> MVKETHRFETFTEEPIRLIGEEGEWLGDFPLDLEGEKLRRLYRDMLAARMLDERYTILIRTGKTSFIAPAAGHEAAQVAIAHAIRPGFDWVFPYYRDHGLALALGIPLKELLGQMLATKADPNKGRQMPEHPGSKALNFFTVASPIASHVPPAAGAAISMKLLRTGQVAVCTFGDGATSEGDWYAGINFAAVQGAPAVFIAENNFYAISVDYRHQTHSPTIADKAHAFGIPGYLVDGMDVLASYYVVKEAVERARRGEGPSLVELRVYRYGPHSSADDDSRYRPKEEVAFWRKKDPIPRFRRFLEARGLWNEEWE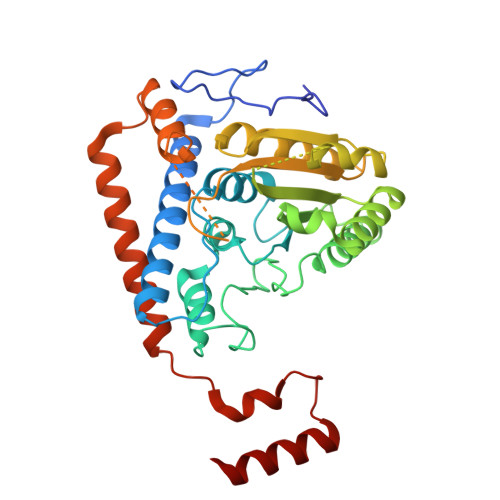EDVREEIRAELERGLKEAEEAGPVPPEWMFEDVFAEKPWHLLRQEALLKEEL> TFPTYKCPETFDAWYCL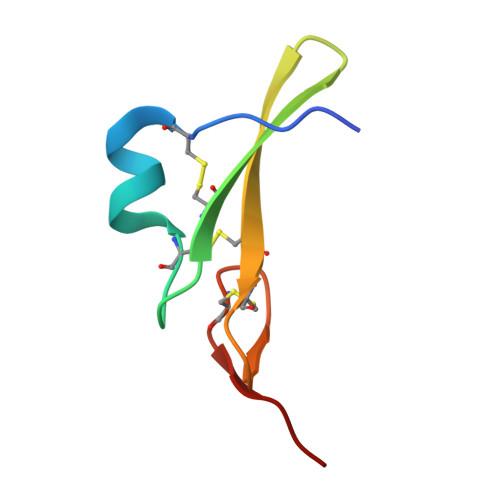NDAHCFAVKIADLPVYSCECAIGFMGQRCEYKEID>MTKENICIVFGGKSAEHEVSILTAQNV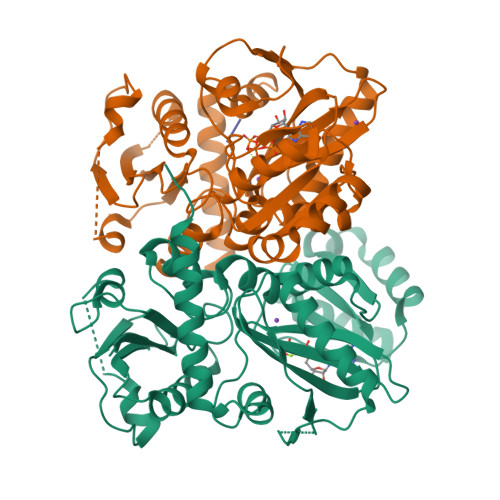LNAIDKDKYHVDIIYITNDGDWRKQNNITAEIKSTDELHLENGEALEISQLLKESSSGQPYDAVFPLLHGPNGEDGTIQGLFEVLDVPYVGNGVLSAASSMDKLVMKQLFEHRGLPQLPYISFLRSEYEKYEHNILKLVNDKLNYPVFVKPANLGSSVGISKCNNEAELKEGIKEAFQFDRKLVIEQGVNAREIEVAVLGNDYPEATWPGEVVKDVAFYDYKSKYKDGKVQLQIPADLDEDVQLTLRNMALEAFKATDCSGLVRADFFVTEDNQIYINETNAMPGFTAFSMYPKLWENMGLSYPELITKLIELAKERHQDKQKNKYKIDRSHHHHHH[2x];> AA> SGISLDNSYKMDYPEMGLCIIINNKNFHKSTGMTSRSGTDVDAANLRETFRNLKYEVRNKNDLTREEIVELMRDVSKEDHSKRSSFVCVLLSHGEEGIIFGTNGPVDLKKITNFFRGDRCRSLTGKPKLFIIQACRGTELDCGIETDSGVDDDMACHKIPVEADFLYAYSTAPGYYSWRNSKDGSWFIQSLCAMLKQYADKLEFM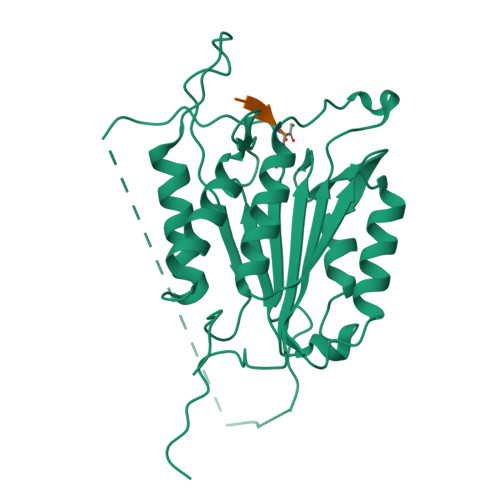HILTRVNRAVATAFESFSFDATFHAKKQIPCIVSMLTKELYFYHH>[2x]GSAKDPAGTAVGLDRALAAITRFGENANNVQNRLGLQENALAQAGDK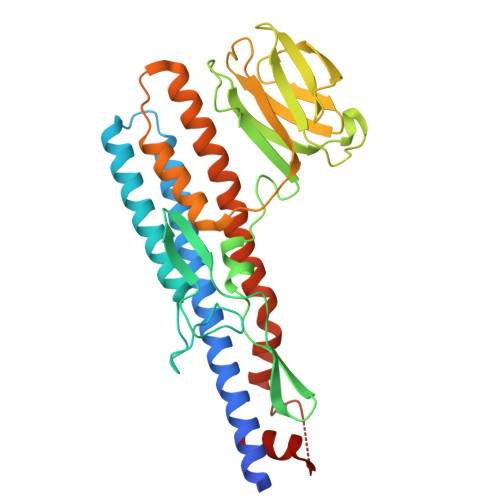MARVTELAVQSNNSSLSPDDRKAIASELTALRDSMVSLANSTDGTGRYLFAGTSDGNAPFIKSNGNVLYNGDQTQKQVEVAPDTFVSDTLPGSEIFMRIRTGDGSVDAHANATNTGTGLLLDFSRDASSGSWNGGSYSVQFTAADTYEVRDSTNALVSTGTYKDGEDINAAGVRMRISGAPAVGDSFQIGASGTKDVFSTIDDMVAALNSDTQTPTQKAAMINTLQSSMRDIAQASSKMIDARASGGAQLSVIDNANSLLESNEVTLKTTLSSIRD4-{[trans-4-({[4-(trifluoromethoxy)phenyl]carbamoyl}amino)cyclohexyl]oxy}benzoic 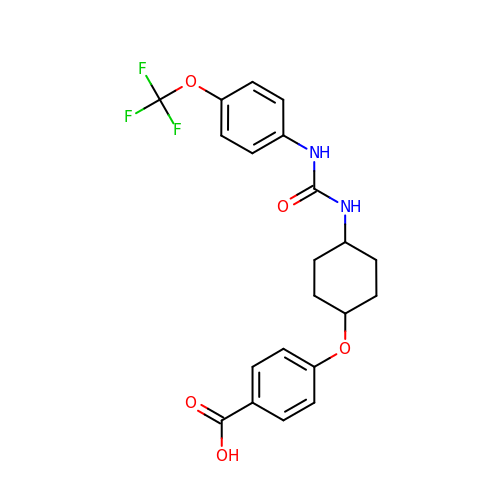acid | C21 H21 F3 N2 O5 | XDVFKCZZXOGEMN-CZIWCDLHSA-N> TKEGYGKHITSMHVRNIFNQGNQVIRNIVKQQRYELLDFTGTEAGTTNLPKIIPYQCIWWRGLQNAANVNQTINNMIALNTISYGVRFLKAKLCIEVYAVTRKRLIQTGATSYYTDDFEQGQNLFIGWADRKAESIPITTPADLDETKLTVANTTLFDANNDNITKEEVPTREKWCHTWDLDVLNHNYLWEPNNLDSQWTLIPGAQAVQPTATPIGPTYQEIVIATKAIGANESALVTTIQDRRSYPRLMLSQPQIKDETDTMKFKYQIRISTELEMEHHIKPDIANPWLTRQTLPLPALSGDGTTRYVPCVPYETHVSQRNWNHVGEYL

We report the discovery of a parvovirus with a bipartite genome, Acheta domesticus segmented densovirus (AdSDV), isolated from house crickets (Acheta domesticus), in which it is pathogenic. Our structural and molecular examinations revealed that the AdSDV packages one genome segment per particle. The AdSDV capsid displayed an overall “smooth” capsid surface with the only protruding area surrounding the fivefold symmetry axis. The AdSDV VP subunit displayed the canonical eight-stranded jelly roll fold, complemented by an N-terminal βA, located on an elongated N-terminal region.

The interior of the FC was filled with density attributed to the ssDNA genome. The vpORF1 sequence could be modeled into the FC density map from Thr47 to Leu377, the final C-terminal residue. To accommodate the density column, the peak of the FC DE loop moves tangentially away from the channel, which is occupied by large aromatic and hydrophobic sidechains, such as Tyr159 and Ile152. The AdSDV is the first parvovirus, where the “density column”, occupying the fivefold channel of the FC fraction, harbors a direct connection to the ordered N-terminus, confirming that N-terminal externalization is a conserved mechanism and independent from the presence of a functional PLA2. The elongated C-terminal portion of the AdSDV-FC proteins enters the capsid interior from the threefold symmetry axis, connecting to the inner surface throughout the twofold interface. Each subunit interacts with the C-terminal tail of the fivefold neighbor to their twofold neighboring subunit. The ordered density of six nucleotides per each FC subunit occupies the interior twofold axis. Five of these are interlinked and interact directly with the capsid surface via π-stacking interactions. The AdSDV FC structure displayed the highest number of ordered nucleotides thus far, which directly interact with the interior capsid surface. This interior-genome interaction, which involves four subunits along with two separate regions of the ssDNA genome, provides additional stability to the otherwise weak interactions at the twofold axis.>[60x]MILAKVTGHVVATQKCDELRGSNLLLITRLDDKQQPMKDQTWVAVDNVGAGMHDIVLAEEYFALNKDRYKAMSVVAIVEKVFRDTEQE;>[180x]MKEALGLIETKGLVACIEAADAMCKAANVELIGYENVGSGLVTAMVKGDVGAVNAAVDSGVEAAKRIGKVVSSRVIARPHNDIEKIAGSTKHKSLRPHNA

Bacterial microcompartments (BMCs) are organelle-like structures consisting of a large quasi-icosahedral or polyhedral protein shell up to 200–300 nm in size and an encapsulated enzymatic core. The glycyl-radical associated microcompartment group 2 (GRM2) type BMC locus encodes the glycyl-radical enzyme-associated microcompartment (GRM) subgroup that includes the choline utilizing locus C (CutC) choline lyase as its signature enzyme. The GRM2 locus therefore contains five structural shell genes encoding four BMC-H proteins and one BMC-P protein. In this study, we demonstrate a practical production system for recombinant GRM2 shell particles from Klebsiella pneumoniae and the requirements for recombinant shell formation.

We analyzed cmcABC′D + CutC336–1128 BDPs with cryo-EM. We calculated a near-atomic (3.3 Å) resolution map for the icosahedral particles and built an atomic model. The particles had a pT = 4 quasi-symmetry with 12 cmcD pentamers occupying the vertices of the icosahedron and 180 BMC-H monomers that were arranged in 30 hexamers within the facets. The map is not of sufficiently high resolution to distinguish between these three types of proteins, so we chose to model cmcC′ in the model, since the mass spectrometry data identified it as the most abundant BMC-H protein in cmcABC′ + D small type particles. The resulting pT = 4 BDP particles are 250 Å in diameter. In the pT = 4 BDP shell, there are three pores: one is in the center of the cmcC′ hexamer, the second is at the threefold axis between the cmcC′ hexamers, and the third is in the center of the cmcD pentamer. The pore in the center of the hexamer is approximately 7 Å in diameter as judged after subtraction of atomic Van der Waals diameters and contains typical GSG pore motifs on the rim. The pore in the center of the cmcD pentamer has a funnel shape and is approximately 16 Å wide on the outer surface but is only approximately 4 Å in diameter on the inner surface as judged by the Van der Waals diameters of atoms forming it. The narrowest part of the pentameric pore is very hydrophobic in nature, as it is lined by tyrosines and phenylalanines. Substrate and cofactor transport across the shell is probably mediated by the largest cmcC′ pore since the other two types of pores are too small or hydrophobic to be involved in this process, if it is assumed that the pores are mostly static in their conformations.>MMKRYLLTLAAFAALGALAQSPTLTIYSGRGQSLVEPLVKQFEAETGIRVQVRYSTDAQILAALQEEGSRSPADLFWANTAGALGQASAKGLLRPLGETLLEKPIAFVPASRTWVPVTVRLRVLAYNPDRIKAEELPESLLDLPRFAREKGLVGRVGWTPTYSSFQDMVAGMIALYGEEKTREWLLAMKALAPKAYPSNPAMLDAIRAGEVDLGSTNHYYVVRFRRAGYRLGMHHFRDGDAGNLALVTGAGLLKTSKNLAAATRFLTYLLSPQAQQYFVGNIGEYPLVKGVALDPNLLPLEEALAKSPKLDLE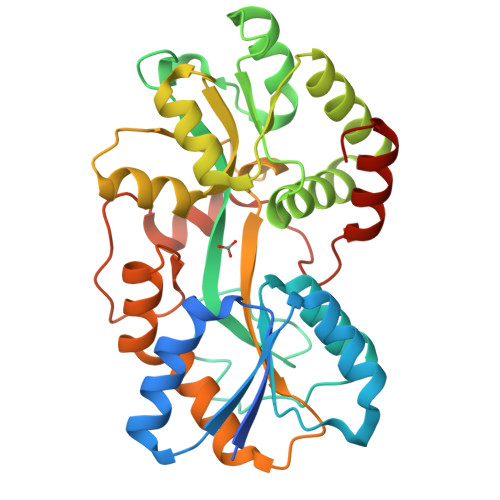KLPLDRALRLLRETGVLHHHHHH[4x]>[2x]MAHHHHHH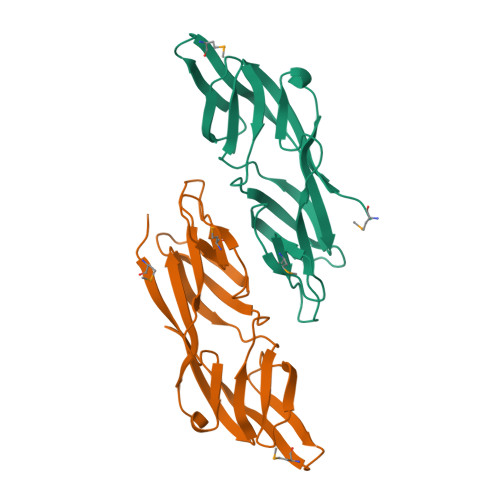MKNTVVRIKAELENVKRLFCDDEYLWIFNIRDSTSSLTRDNIQFRKTDILEIPNSRGTANFMIKWTEYPKYSTINFVNTKNSCSYEEVNNNEWRDFASFECRGIELIDFFPSNNFIVEDTKGKLYYDVNLSDQNWCDYNEEHEMCVGIYNLEYEVN>GPGSSENRNRKLSYQEYYVDGDYEEVRKKLPEIIKQARIKASQVMEPTIYEKRVVMEIIKDFIRDKGRKVYGGTALNETIKKKNPEDAIYDSYLFSDIEFYSPTPVPDLKELCDILYHKGYDPVQGKEAQHEETYSIFVNLQLYCDITYVPTKVYHGIKTIEIDGINYTHPHFMLIDYLRMINQPLTAAEQRWEKAFDRMYVLLKNYPMEKYDNSMRITSPRDDIQMYIGKVKSEFMKIPEIQESCLISGFDAYNFFIRHAMGDRKVEQMARIKNDYNSLKNFITVLPFMELISVKYKDTVEKLYNFLREKVVNPDLITIDEYFPLFQFTGYSVSINYDGIPIVKVYEADGYCVPDIKTTSGYRYVSYQYILMIMYISKFKAHLDKNKEMYFNYGIAISNLVQARNSYLNQKNIGVINDTVFSEFRIGCIGTTVSYTRMSRLRMLEKKKQGKVIQFVYTPKQYFSQTPEQQNNFDESMKKYRFKNTSGNKIT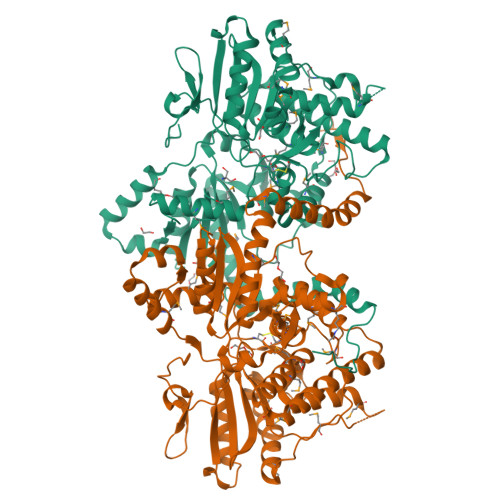IPKNLLFKIDERGNISEEISTEEAYITEDTTSINTTTDINTN[2x]> SPIRHVTPHLSHSTPIPRDMQGNSSQSPNTPWQGYDINTNYYETIPQTNVVREYWFDIVNTTAALDGVERPVLLVNGQFPGPTIEANWGDTVKVHVTNRMENNGTAIHFHGIRQLYNNQMDGVAALTQCPVPPNSSYTYVWRAEEYGSSWYHSHFSLQAWEGVFGGILIHGPSTAEYDHDLGMVFLNDWSHQTVDEMYQSVLESQNPPHFQTGLINGSNIWVTADNQTVGRRFQTEFVPGQRYRLRLVNAAMDTHFRFSIDNHDLTVIASDFVPIVPFTTNNVPIGMGQRYDIIVTANQAPDNYWIRAIPQSFCSDNANSDNIKGVLHYEGAADNSDPTSTKWDYGDDIQCLDFSLDELVPWLALDADIGG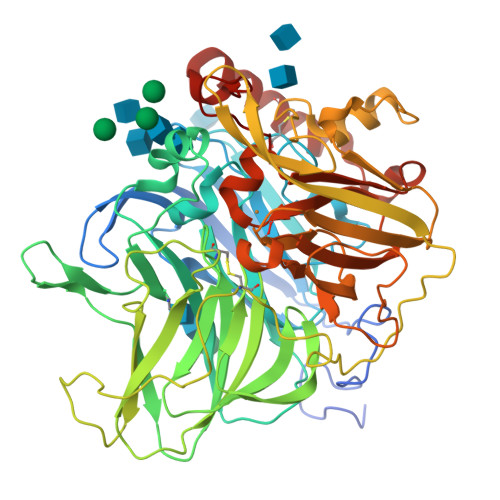AQMAESDVDFTPFGDVPLYLWTMGGNALNISWKDPTLQQTFEDPDKMDWKASQGVIEAAIPNKWTVLVVQTDLPVPHPIHLHGHDFYLLAQGFGQFNPQNVTLKTHNPPRRDTALMTAATPENGGGGYMVIGFPADNPGVWLIHCHIGFHATEGFAQQIVERQSEFNTFFSEDLLENTCDAWDEYAKVNPYGHQYRALAGPYESGI> RNKPGKATGKGKPVNNKWLNNAGKDLGSPVPDRIANKLRDKEFKSFDDFRKKFWEEVSKDPELSKQFSR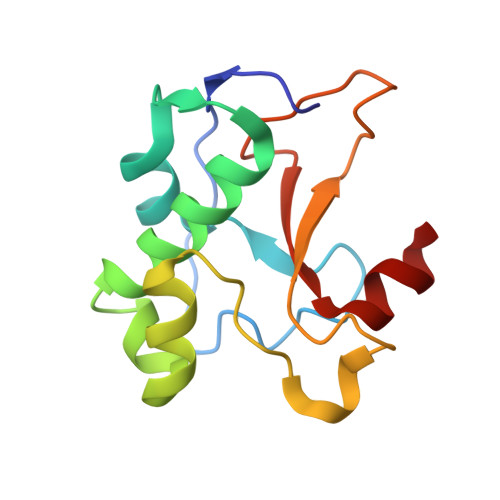TQNDRMKVGRAPQTRTQDVSGKRQSFELHHEKPISQNGGVYDMDNISVVTPKRHIDIH Picobirnaviruses (PBV) are small, non-enveloped dsRNA viruses infecting a wide range of mammalian and avian species. Human PBV (hPBV) has been identified on almost every continent, and has been associated with acute gastroenteritis primarily in children and people that are immunocompromised. It has a bi-segmented genome with the genome segment two (PBV2) encoding the viral RdRP and the genome segment one (PBV1) encoding the CP and a protein of unknown function. The hPBV RdRP possesses a canonical polymerase fold with a 24 amino acids (aa) long C-terminal insertion loop structure that partially occupies the active site of the polymerase. The polymerase domain, which is structurally highly conserved amongst RNA viruses, has a right-hand configuration with three subdomains: the fingers (aa 85–230, 268–324), palm (aa 231–267, 325–414), and thumb (aa 415–470).

The purified hPBV RdRP (534 aa, ~62 kDa with a N-terminal 6xHis tag) exists in solution as a monomer, based on its gel filtration chromatography elution profile. hPBV RdRP was crystallized in the space group of P21 with two molecules in each asymmetric unit. The crystal structure was solved to 2.4 Å resolution by single-wavelength anomalous dispersion (SAD) using Se-Met derivatized crystals. In the final model of the hPBV RdRP, one molecule is comprised of residues 1–494, 500–511, and 518–534, while the other molecule contains residues 1–495 and 520–534. The polypeptide can be divided into three domains based on their function: an N-terminal domain (aa 1–84), a core polymerase domain (aa 85–470), and a C-terminal domain (aa 471–534). The palm subdomain hosts the three key aspartic acid residues, D261, D359, and D360, of the active site. The hPBV RdRP contains three channels leading to the active site of the protein that are believed to allow for dsRNA product export, template entry and NTP uptake. The hPBV RdRP possesses a highly flexible, 24-aa insertion loop structure (aa 495–518) formed by an internal sequence from the C-terminal domain. This loop structure, which is associated with higher than average temperature factor values, extends from the C-terminal domain towards the catalytic site. In this model, the 3’-end of the template collides with the hPBV insertion loop structure, suggesting that the insertion loop in its current position would sterically prevent the template from binding to the active site of the RdRP as expected in the assembly of a productive initiation complex (right). Therefore, the hPBV insertion loop structure must undergo a significant conformational change in order for RNA binding and replication to take place.

>[2x]GQVAPNVWSKYFNIPNPGLRAYFSNVVSGQPEVYRTPFYKGMSLESICDEWYKKLVSIDTQWPTLMEFEDDLRKKVGPMSVMLPLKERMSDIDSYYDSISKDQVPFDTKAISAAKSEWKGVSRLRLRSEVNTVAVMKKSTNSGSPYFSKRKAVVSKTIPCDVYMDGRYCVMRQNGREWSGAAVLGWRGQEGGPKPTDVKQRVVWMFPFAVNIRELQVYQPLILTFQRLGLVPAWVSMEAVDRRITKMFDTKGPRDVVVCTDFSKFDQHFNPTCQSVAKELLADLLTGQEAVDWLERVFPIKYAIPLAYNWGEIRYGIHGMGSGSGGTNADETLVHRVLQHEAAISHHTTLNPNSQCLGDDGVLTYPGISAEDVMQSYSRHGLDMNLEKQYVSKQDCTYLRRWHHTDYRVDGMCVGVYSTMRALGRLAMQERYYDPDVWGEKMVTLRYLSIIENVKYHPLKEEFLDFCIKGDKTRLGLGIPGFLDNIAGEAQKAIDMMPDFLGYTKSLQYDGDLRRNAAAGIENWWVVQALKSRR>[2x]MASMTGGQQMGRGSEFMIASVRGEVLEVALDHVVIEAAGVGYRVNATPATLATLRQGTEARLITAMIVREDSMTLYGFPDGETRDLFLTLLSV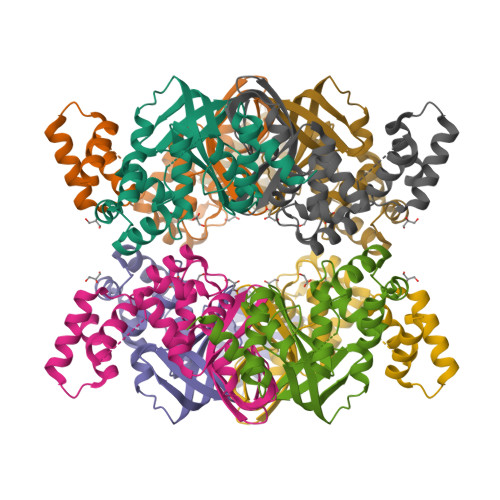SGVGPRLAMAALAVHDAPALRQVLADGNVAALTRVPGIGKRGAERMVLELRDKVGVAATGGALSTNGHAVRSPVVEALVGLGFAAKQAEEATDTVLAANHDATTSSALRSALSLLGKAR> AER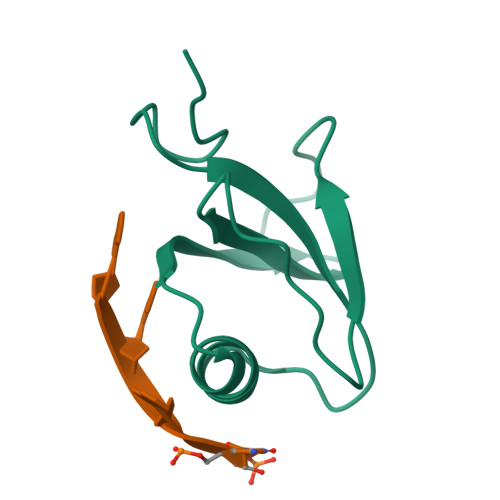SLLTGEEGWRTYKATGPRLSLPRLVALLKGQGLEVGKVAEAEGGFYVDLRPEARPEVAGLRLEPARRVEGLLEIPSRTRRPARA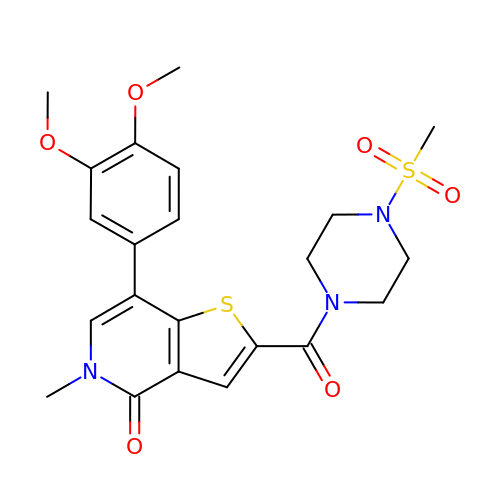7-(3,4-dimethoxyphenyl)-5-methyl-2-(4-methylsulfonylpiperazin-1-yl)carbonyl-thieno[3,2-c]pyridin-4-one | C22 H25 N3 O6 S2 | BEIFGZXXCPXAAY-UHFFFAOYSA-N> MATFTTEQAGYQMQAILQVIGYDLLIVVTGGTNPHIGDVTTLTASTVPETVKFPSHDGRFHKDNFISERMAKRIQRYLAGSCTITAGIHVNQITKAQIAAAAPMTDDLSRQIISWLQAHPVQAEKPEYYGQDEQPR

Previous studies indicated that the small protein LpdD (lp_0272) is associated with the UbiD-type gallate decarboxylase LpdC (lp_2945) in Lactobacillus plantarum. The crystal structure of the purified LpdD reveals a dimeric protein with structural similarity to the eukaryotic heterodimeric proteasome assembly chaperone Pba3/4. Solution studies demonstrate that LpdD protein specifically binds to reduced prFMN species only. The addition of the LpdD–prFMNH2 complex supports reconstitution and activation of the purified E. coli apo-UbiD in vitro, leading to modest 3,4-dihydroxybenzoic acid decarboxylation. These observations suggest that LpdD acts as a prFMNH2-binding chaperone, enabling apo-UbiD activation through enhanced prFMNH2 incorporation and subsequent oxidative maturation.

Given both H35 and H61 are strictly conserved, we made LpdD H35A and H61A variants to test for the effect of an intact metal-binding site on prFMNH2 binding. In the case of the H35A variant, crystals belonged to a different space group (P41212) containing only one molecule in the asymmetric unit. As with the WT structure, a functional and highly similar dimer can be made by applying crystallographic symmetry. The H35A monomer superposed with rmsd of 0.35 Å to the Mn2+-bound WT LpdD, with significant conformational changes observed in loops spanning 8 to 11, 30 to 36, 54 to 62, and 89 to 95 encompassing most of the strictly conserved residues. No electron density for Mn2+ could be observed, but residual electron density was observed and assigned to a bound phosphate near H61. While the distinct crystallization conditions and crystal packing likely contribute to the observed changes, it is clear the presence of H35 is essential for metal binding and associated loop conformations. When tested using whole-cell decarboxylation assays, both variants displayed reduced activity when compared with WT LpdD whole-cell assays, with H35A more affected than H61A. In vitro reconstitution of the purified H61A variant reveals this mutation does not abolish prFMNH2 binding, whereas the purified H35A variant did not bind prFMNH2 under the conditions used. This suggests that His35—and by extension metal binding—is more important for LpdD function in vivo compared with H61, although neither are essential under the conditions tested.>MLLEAIFHEAKGSYAYPISETQLRVRLRAKKGDVVRCEVLYADRYASPEEELAHALAGKAGSDERFDYFEALLECSTKRVKYVFLLTGPQGEAVYFGETGFSAERSKAGVFQYAYIHRSEVFTTPEWAKEAVIYQIFPERFANGDPSNDPPGTEQWAKDARPRHDSFYGGDLKGVIDRLPYLEELGVTALYFTPIFASPSHHKYDTADYLAIDPQFGDLPTFRRLVDEAHRRGIKIILDAVFNHAGDQFFAFRDVLQKGEQSRYKDWFFIEDFPVSKTSRT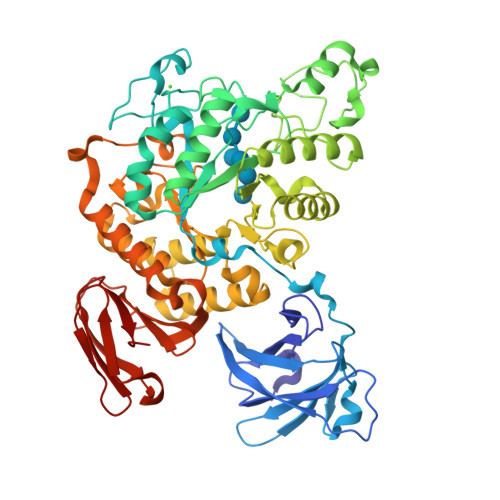NYETFAVQVPAMPKLRTENPEVKEYLFDVARFWMEQGIDGWRLNVANEVDHAFWREFRRLVKSLNPDALIVGEIWHDASGWLMGDQFDSVMNYLFRESVIRFFATGEIHAERFDAELTRARMLYPEQAAQGLWNLLDSHDTERFLTSCGGNEAKFRLAVLFQMTYLGTPLIYYGDEIGMAGATDPDCRRPMIWEEKEQNRGLFEFYKELIRLRHRLASLTRGNVRSWHADKQANLYAFVRTVQDQHVGVVLNNRGEKQTVLLQVPESGGKTWLDCLTGEEVHGKQGQLKLTLRPYQGMILWNGR[2x]>[6x]GGGGGGMKLFKELEETKEQVIKMAKLVQEAIDKATEALNKQNVELAEEVIKGDDTIDLLEVDIERRCIRMIALYQPEAGDLRMIMGIYKIVSDLERMGDEAENIAERAILLAEEPP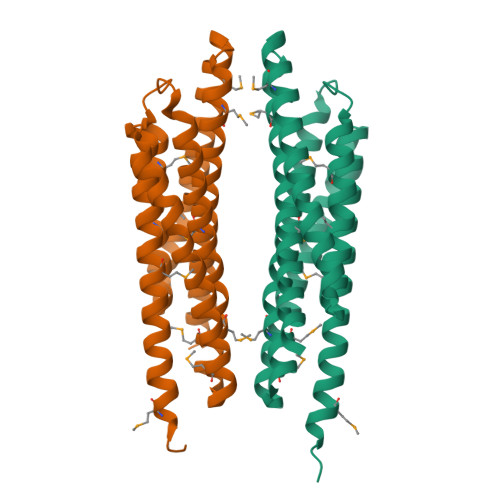LKPYVNINFMSEIVKEMVNDSVISFIQQDTLLAKKVIEKDDTVDELYHQLERELMTYVLEDPRNIKRAMHLSFVARHYERIADHAENVAEAAIYLSEGEIVKHQHIKEKGE>[3x]HHHHHHGLIQERRSHEVNPAAHLTGANSSLTGSGGPLLWETQLGLAFLRGLSYHDGALVVTKAGYYYIYSKVQLGGVGCPLGLASTITHGLYKRTPRYPEELELLVSQQSPCGRATSSSRVWWDSSFLGGVVHLEAGEEVVVRVLDERLVRLRDGTRSYFGAFMV;>INITSSASQEGTRLNLICTVWHKKEEAEGFVVFLCKDRSGDCSPETSLKQLRLKRDPGIDGVGEISSQLMFTISQVTPLHSGTYQCCARSQKSGIRLQGHFFSILFTETGNYTVTGLKGGGGSGGGGSGGGGSGGGGSLPSCKEDEYPVGSECCPKCSPGYRVKEACGELTGTVCEPCPPGTYIAHLNGLSKCLQCQMCDPAMGLRASRNCSRTENAVCGCSPGHFCIVQDGDHCAACRAYATGHHHHHH[3x]

HVEM is a TNF (tumor necrosis factor) receptor contributing to a broad range of immune functions involving diverse cell types. It interacts with a TNF ligand, LIGHT, and immunoglobulin (Ig) superfamily members BTLA and CD160. HVEM engages in bidirectional signaling, serving not only as a receptor but also as a ligand for IgSF receptor signaling. To dissect the molecular basis for multiple functions, we determined crystal structures that reveal the distinct HVEM surfaces that engage LIGHT or BTLA/CD160, including the human HVEM–LIGHT–CD160 ternary complex, with HVEM interacting simultaneously with both binding partners.

The asymmetric unit contains three copies of each hHVEM, hLIGHT, and hCD160, forming a ternary complex with 3:3:3 stoichiometry. Within the ternary assembly, hHVEM and hLIGHT exhibit the classical 3:3 TNF–TNFR assembly, with contacts that are very similar to the structure of the hHVEM–hLIGHT binary complex described above. The hHVEM–hLIGHT complex forms the core of the ternary complex, with each hHVEM CRD1 further binding a single molecule of hCD160 in a manner similar to that observed in the structure of the hHVEM–hCD160 binary complex. Notably, the structures of hHVEM–hLIGHT–hCD160 and hHVEM–hCD160 complexes relied on the use of a single chain hCD160–hHVEM fusion protein, as the relatively weak interaction of hCD160–hHVEM (7.1 ± 0.9 µM) does not support the stable complex formation in solution. The crystal structure of the hHVEM–hLIGHT–hCD160 complex provides direct evidence that hLIGHT and hCD160 can simultaneously engage hHVEM, resulting in a higher-order assembly with the potential of coordinated signaling through both hHVEM and hCD160. Notably, the simultaneous interaction of hCD160 and hLIGHT with hHVEM alters the local organization of hCD160, as engagement of hHVEM with trimeric hLIGHT may enforce close proximity of up to three hCD160 molecules with distinct geometric organization, as compared with the engagement of hCD160 and hHVEM in the absence of hLIGHT. Crystal structures of hHVEM in complex with hBTLA and hCD160 highlight an anti-parallel intermolecular β-strand interaction, in which the β-strand composed of residues G72-P77 from CRD1 in hHVEM contacts the edge β-strands in hBTLA and hCD160 through canonical main-chain-to-main-chain β-sheet hydrogen bonds. This pattern of hCD160 interactions with hHVEM is conserved in the ternary hHVEM–hLIGHT–hCD160 complex. The recognition interfaces in the ternary hHVEM–hLIGHT–hCD160 complex are similar to those in the binary hHVEM–hCD160 and hHVEM–hLIGHT complexes, suggesting that little molecular accommodation is required for HVEM to simultaneously engage two types of binding partners. Because both hCD160 and hBTLA bind to similar epitopes on hHVEM CRD1, it is likely that hHVEM, hLIGHT, and hBTLA are able to form a ternary complex similar to the trimolecular complex of hHVEM–hLIGHT–hCD160 we have determined.> DF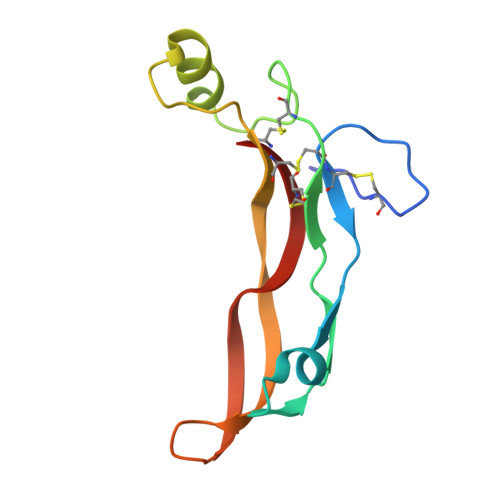GLDCDEHSTESRCCRYPLTVDFEAFGWDWIIAPKRYKANYCSGECEFVFLQKYPHTHLVHQANPRGSAGPCCTPTKMSPINMLYFNGKEQIIYGKIPAMVVDRCGCS>MSLIEERLKHYLEKQIPARDQYIEQMEREAHEQQVPIMDLLGMESLLHLLKMAAPARILEIGTAIGYSAIRMAQALPEATIVSIERDERRYEEAHKHVKALGLESRIELLFGDALQLGEKLELYPLFDVLFIDAAKGQYRRFFDMYSPMVRPGGLILSDNVLFRGLVAETDIEHKRHKQLATKIDTYNQWL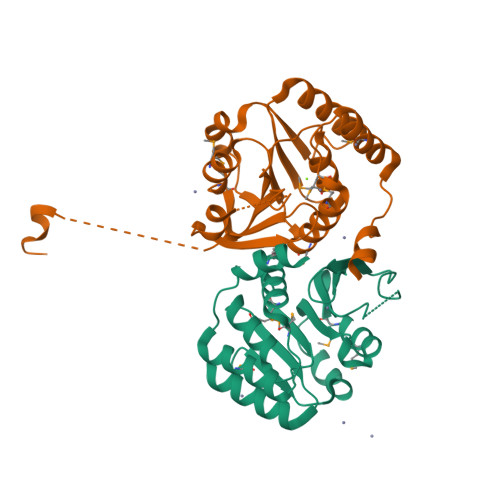LEHPQYDTRIFPVGDGIAISIKRETKGDTDDEKAEGHHHHHH[2x]(2R,3S,4R)-3-(2',6'-difluoro-4'-methyl[1,1'-biphenyl]-4-yl)-4-(fluoromethyl)azetidine-2-carbonitrile 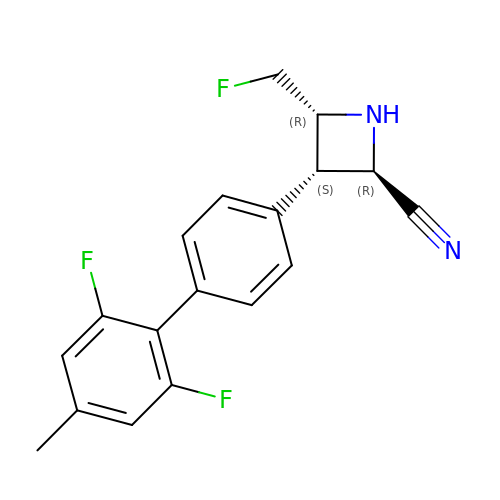| C18 H15 F3 N2 | OZFKPHFHTNQIQS-XYJFISCASA-N k-Turns are widespread RNA architectural elements that mediate tertiary interactions. The standard k-turn is formed in duplex RNA where a short bulge is followed by G·A and A·G basepairs, and folds to generate a kink with an included angle of 50° between the axes of the two helical arms. We describe a double-kink-turn motif comprising two inverted k-turns that forms a tight horse-shoe structure that can assemble into a variety of shapes by coaxial association of helical ends. Using X-ray crystallography we show that these assemble with two (dumbell), three (triangle) and four units (square), with or without bound protein, within the crystal lattice.

We therefore considered the possibility that if three two-k-turn units were contained within the same double-stranded molecule this might fold to generate a closed quasi-continuous triangular species. We synthesized the 114 nt self-complementary RNA shown in Fig. 4A. The 3′ cytosine nucleotides of the two-k-turn units were changed to uridine, so that the connected NC helices contain central U·G and G·U pairs. The RNA was crystallized in the absence of protein. The ends of the RNA have associated by coaxial stacking. This is so perfect that these non-covalent ends are randomly located within the crystal lattice, i.e. there is a crystallographic three-fold rotational axis through the centre perpendicular to the plane of the triangle. The overall shape of the six-k-turn object that has been effectively cyclized by crystal symmetry is a triangle with edges defined by the C helices and vertices formed by the NC helices. The overall structure is therefore reminiscent of the chair form of cyclohexane but with RNA helices in place of carbon–carbon bonds.

> GGCGAAGAACU;> GGGGAGCU>MKPYDLSEAVAVVTGGSSGIGLATVELLLEAGAAVAFCARDGERLRAAESALRQRFPGARLFASVCDVLDALQVRAFAEACERTLGCASILVNNAGQGRVSTFAETTDEAWSEELQLKFFSVIHPVRAFLPQLESRADAAIVCVNSLLASQPEPHMVATSAARAGVKNLVRSMAFEFAPKGVRVNGILIGLVESGQWRRRFEAREERELDWAQ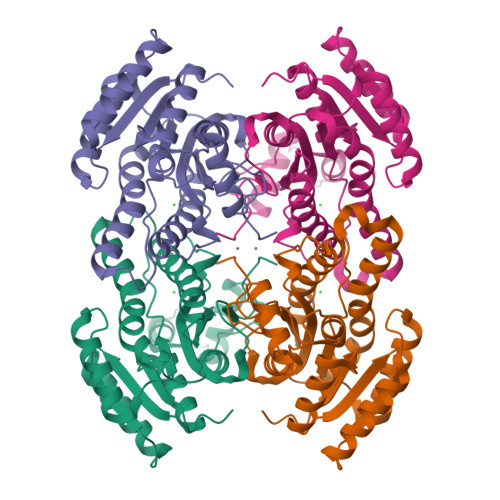WTAQLARNKQIPLGRLGKPIEAARAILFLASPLSAYTTGSHIDVSGGLSRHA[2x]> ETDEEPEEPGRRGSFVEMVDNLRGKSGQGYYVEMTVGSPPQ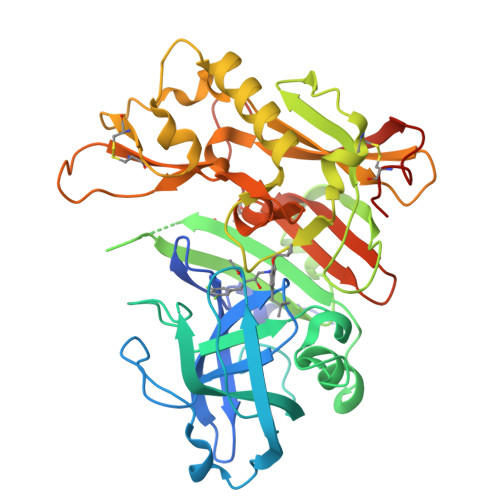TLNILVDTGSSNFAVGAAPHPFLHRYYQRQLSSTYRDLRKGVYVPYTQGAWAGELGTDLVSIPHGPNVTVRANIAAITESDKFFINGSNWEGILGLAYAEIARPDDSLEPFFDSLVKQTHVPNLFSLQLCGAGFPLNQSEVLASVGGSMIIGGIDHSLYTGSLWYTPIRREWYYEVIIVRVEINGQDLKMDCKEYNYDKSIVDSGTTNLRLPKKVFEAAVKSIKAASSTEKFPDGFWLGEQLVCWQAGTTPWNIFPVISLYLMGEVTNQSFRITILPQQYLRPVEDVATSQDDCYKFAISQSSTGTVMGAVIMEGFYVVFDRARKRIGFAVSACHVHDEFRTAAVEGPFVTLDMEDCGYNIPQTDES>MVNPAERLAELDGVLMQYLLEADLLRELPPTYRLVLLPLDEPEVAAQALAWAMEAPNPEGWPSVYALFLQGR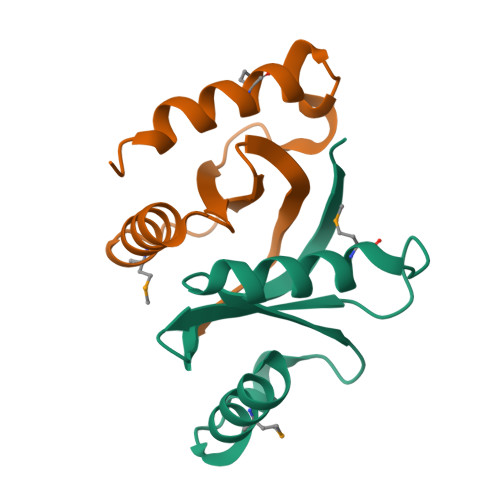PIRLLLLGKEVEVAPRAA[2x]>MKPYIRRGGRPGDETYYLNIPRDIAKALGITKEDEFMLSVETKDGEITLCYKR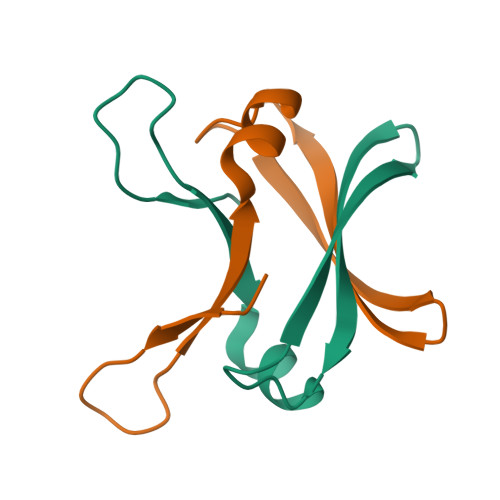VKK[2x]>[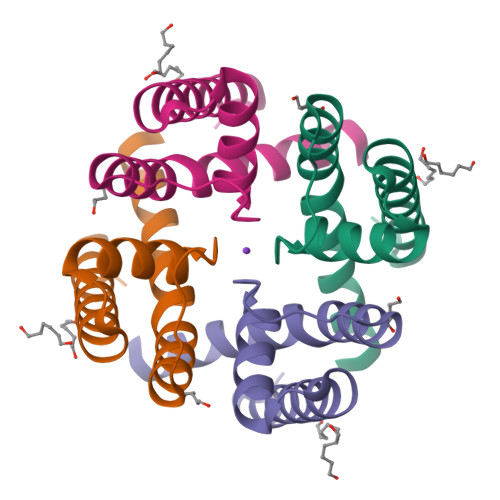8x]HLPRVLKVPATRILLLVLAVIIYGTAGFHFIEGESWTVSLYWTFVTIATVGYGDYSPHTPLGMYFTCTLIVLGIGTFAVAVERLLEFLINR> SDSRTVSEPKTPSSCTTLKADSSTATSTIQKALNNCDQGKAVRLSAGSTSVFLSGPLSLPSGVSLLI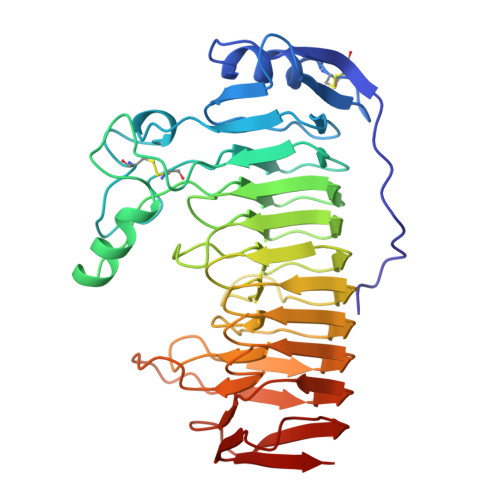DKGVTLRAVNNAKSFENAPSSCGVVDKNGKGCDAFITAVSTTNSGIYGPGTIDGQGGVKLQDKKVSWWELAADAKVKKLKQNTPRLIQINKSKNFTLYNVSLINSPNFHVVFSDGDGFTAWKTTIKTPSTARNTDGIDPMSSKNITIAYSNIATGDDNVAIKAYKGRAETRNISILHNDFGTGHGMSIGSETMGVYNVTVDDLKMNGTTNGLRIKSDKSAAGVVNGVRYSNVVMKNVAKPIVIDTVYEKKEGSNVPDWSDITFKDVTSETKGVVVLNGENAKKPIEVTMKNVKLTSDSTWQIKNVNVKK>SNAGMTGFVINTRRAPFDDWRLREALLLAFNFEFINDTVTGGVMPRITSYFSGTDLAYRPGTASGREAELLAPFAADLPPGTLEGYALPQGDG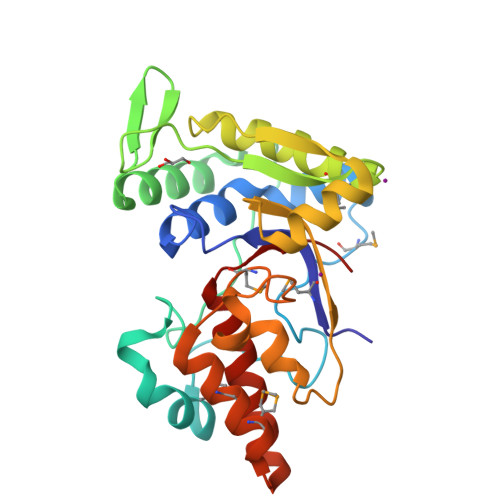TARNRTNLRRAAQFLEQAGFRIEQGQLLGPDGAPLALRFLLRQGDSDMQTVLEIYTRALERLGIAAQIEKVDNAQYTARVAELDFDLTPFRRDLSLSPGNEQRLYWGSHSAGQPGTRNLMGAASPAIDAMIDRMLAATTEDELTAATRALDRVLTAGRYVIPIWR[4x]>MPHRFKVYNYMSPTFCDHCGSLLWGLVKQGLKCEDCG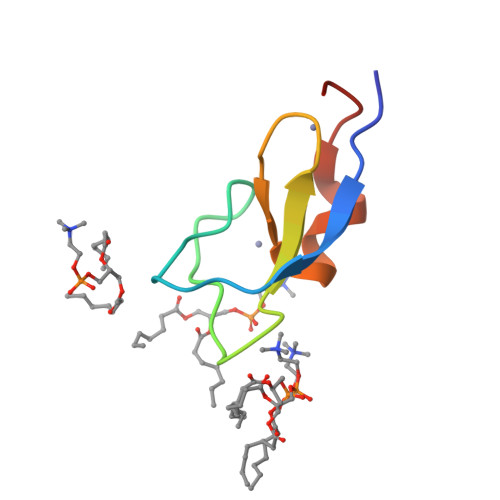MNVHHKCREKVANLCG[2x]> PKHEFSVDMTCGGCAEAVSRVLNKLGGVKYDIDLPNKKVCIESEHSMDTLLATLKKTGKTVSYLG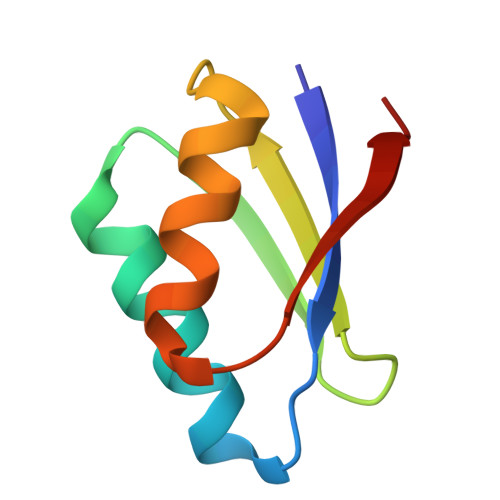LEI>SMSHYKSNVRDQVFNLFEVFGVDKVLGADKFSDLDADTAREMLTEIARLAEGPIAESFVEGDRNPPVFDPETHTVTLPEGFKKSMRALFDGGWDKVGLAEHLGGIPMPRALQWALIEHILGANPAAYMYAMGPGMSEIFYNNGTDEQKKWATIAAERGWGATMVLTEPDAGSDVGAGRTKAVQQPDGTWHIEGVKRFITSADSDDLFENIMHLVLARPEGAGPGTKGLSLFFVPKFHFDHETGEIGERNGVFVTNVEHKMGLKVSATCELSLGQHGIPAVGWLVGEVHNGIAQMFDVIEQARMMVGTKAIATLSTGYLNALEYAKERVQGADMTQMTDKTAPRVTITHHPDVRRSLMTQKAYAEGLRAIYLYTATFQDAEVAQAVHGVDGDLAARVNDLLLPIVKGFGSETAYAKLTESLQTLGGSGFLQDYPIEQYIRDSKIDSLYAGTTAIQAQDFFFRKIIRDKGQALAYVAGEIEQFIKNENGNGRLKTERELLATALADVQGMAASLTGYLMAAQEDAASIYKVGLGSVRFLMAVGDLLSGWLLARQAAVAIEKLDAGATGADKSFYEG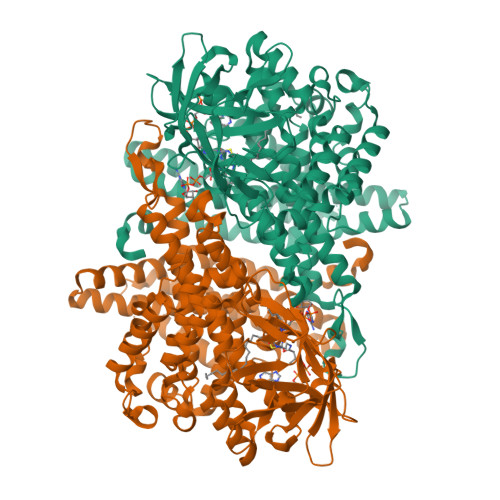KIAAASFFAKNMLPLLTSTRQIIENLDNDVMELDEAAF[2x]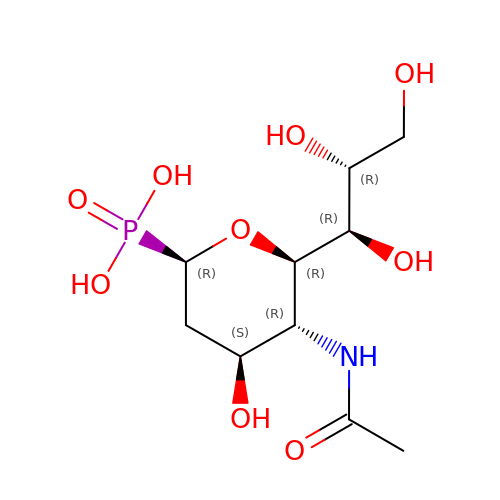(1R)-4-acetamido-1,5-anhydro-2,4-dideoxy-1-phosphono-D-glycero-D-galacto-octitol | C10 H20 N O9 P | QITAGYVZDNZULE-IHICSVBISA-N> SLDVLIVYELTPTVEEKAKADTLKLPPTFFCYKNRPDYVSEEEEDDEDFETAVK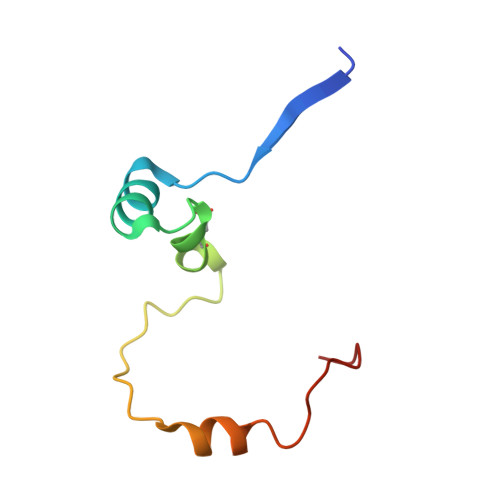KLNGKLYLDGSEK Tyrosine hydroxylase (TH) catalyzes the rate-limiting step in the biosynthesis of dopamine (DA) and other catecholamines, and its dysfunction leads to DA deficiency and parkinsonisms. Mammalian AAAHs mainly present as homotetramers with a three-domain subunit structure: an N-terminal regulatory domain (RD) that consists of a structured ACT (aspartate kinase-chorismate mutase-TyrA) domain preceded by a less structured N-terminal tail of varying length; a central catalytic domain (CD) that contains the active site iron and binding-sites for substrate and cofactor; and a C-terminal oligomerization domain (OD) responsible for dimerization and/or tetramerization. Inhibition by catecholamines and reactivation by S40 phosphorylation are key regulatory mechanisms of TH activity and conformational stability. We used Cryo-EM to determine the structures of full-length human TH without and with DA, and the structure of S40 phosphorylated TH, complemented with biophysical and biochemical characterizations and molecular dynamics simulations.

We were only able to rigid-body fit a good-quality homology model (82% identity) into the lower resolution RD density. This explains the lower quality of the RD fitting in comparison with the atomic resolution modeling of the CD. For this reason, we built a model in which the side chains were omitted from the RD structure. In our structural model of TH(DA), S40 was placed on the N-terminal side of the α-helix, at the base of the active site. Finally, two of the apo-TH-specific peptides reflected an interaction between the N-terminus of the protein and K204, a residue found in an external α-helix that surrounds the active centre. The larger number of crosslinks involving the N-terminus in apo-TH compared with TH(DA) speaks of a higher flexibility of the former, which is consistent with the presence of an immobile α-helix in the latter that would limit the movement of the entire N-terminal tail, indicative of increased protein stability. As DA-mediated TH stabilization largely determines the steady-state levels of TH and DA in vivo, the full-length TH(DA) structure obtained in this work improves our understanding of the structure-based pathogenic mechanism in THD.

>[4x]SLIEDARKEREAAVAAAAAAVPSEPGDPLEAVAFEEKEGKAMLNLLFSPRATKPSALSRAVKVFETFEAKIHHLETRPAQRPRAGGPHLEYFVRLEVRRGDLAALLSGVRQVSEDVRSPAGPKVPWFPRKVSELDKCHHLVTKFDPDLDLDHPGFSDQVYRQRRKLIAEIAFQYRHGDPIPRVEYTAEEIATWKEVYTTLKGLYATHACGEHLEAFALLERFSGYREDNIPQLEDVSRFLKERTGFQLRPVAGLLSARDFLASLAFRVFQCTQYIRHASSPMHSPEPDCCHELLGHVPMLADRTFAQFSQDIGLASLGASDEEIEKLSTLYWFTVEFGLCKQNGEVKAYGAGLLSSYGELLHCLSEEPEIRAFDPEAAAVQPYQDQTYQSVYFVSESFSDAKDKLRSYASRIQRPFSVKFDPYTLAIDVLDSPQAVRRSLEGVQDELDTLAHALSAIG> GTLTGERPPVFWLQGQGCTGCSVTLLNSVHPSIADVLLKVISLEFHPTVMAWEGEHAIEHMRKVAEKFKGKFFLVIEGSVPVEADGKYCIIGEANHHEISMVDALKEFGPNAAAVLAVGTCAAYGGIPAAEGSETGATAVSKFLGDNGIKTPVVNIPGCPPHPDWIVGTVVLALDAIKKNGLEGGLAEVVKVLDSDGRPTPFFGRNIHENCPYLDKYDEGVMSATFTDKVGCRYDLGCKGPMTMADCFERKWNGGVNWCVQNAVCIGCVEPDFPDGKSPFYQA;> GATGRTTIAIDPVTRIEGHLKAEVVVENGKVVDARLSGGMYRGFETILRGRDPRDASQIVQRICGVCPTAHSTASVLALDEAFGAKVPNNGRITRNLIFGANYLQSHILHFYHLSAQDFVQGPDTAPFVPRFPKSDLRLSKELNKAGVDQYIEALEVRRICHEMVALFGGRMPHVQGQVVGGATEIPTKEKLVEYAARFKKVRDFVEQKYVPVVYTIGSKYKDMFKVGQGFKAALCVGAFPLDNSGKKHLFMPGVYAKGKDMPFDPSKIKEYVKYSWFAEETTGLNYKEGKTIPAPDKAGAYSFVKAPRYDGLSLEVGPLARMWVNNPELSPVGKKLLKDLFGISAKKFRDLGEEAAFSLMGRHVARAEETYYMLGAIEGWLKEIKAGEDTVVMPAVPASAEGTGFTEAPRGSLLHYVKVKDSK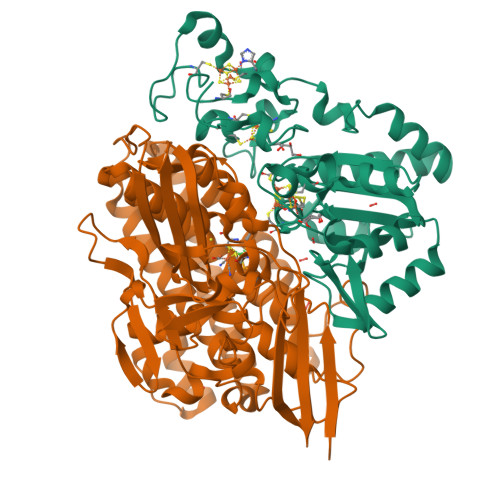IDNYQIVSASLWNCNPRDDMGQRGAVEEALIGIPVDDIQNPVNVARLIRAFDPULACAVH> STQEQTPQICVVGSGPAGFYTAQHLLKHHSRAHVDIYEKQLVPFGLVRFGVAPDHPEVKNVINTFTQTARSDRCAFYGNVEVGRDVTVQELQDAYHAVVLSYGAEDHQALDIPGEELPGVFSARAFVGWYNGLPENRELAPDLSCDTAVILGQGNVALDVARILLTPPDHLEKTDITEAALGALRQSRVKTVWIVGRRGPLQVAFTIKELREMIQLPGTRPMLDPADFLGLQDRIKEAARPRKRLMELLLRTATEKPGVEEAARRASASRAWGLRFF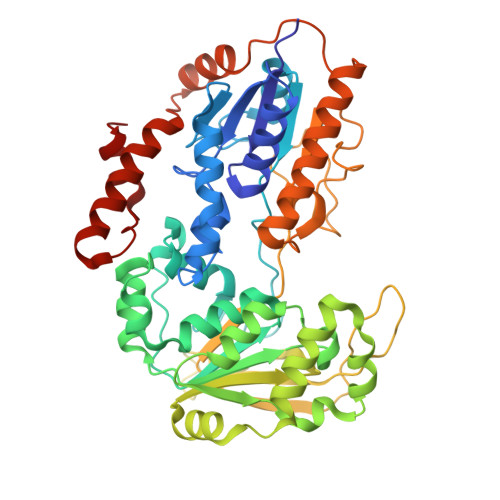RSPQQVLPSPDGRRAAGIRLAVTRLEGIGEATRAVPTGDVEDLPCGLVLSSIGYKSRPIDPSVPFDPKLGVVPNMEGRVVDVPGLYCSGWVKRGPTGVITTTMTDSFLTGQILLQDLKAGHLPSGPRPGSAFIKALLDSRGVWPVSFSDWEKLDAEEVSRGQASGKPREKLLDPQEMLRLLGH>[2x]GVTDNPRELQVKYLTTYQKDEEKLSA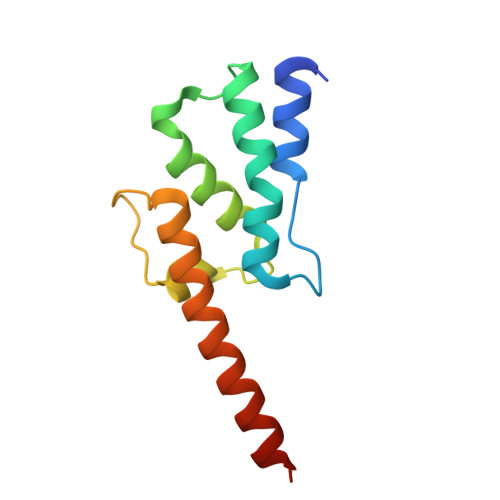YVLRLEPLLQKLVQRGAIERDAVNQARLDQVIAGAVHKTIRRELNLPEDGPAPGFLQLLVLIKDYEAAEEEEALLQAILEGNFT> MKYNAPNTTPSSIGPQIRLDYYYKKALVDAAKEMYFGQLAEVTNMPKNMGKQIKLYHYVPLLDDRNVNDQGIDAAGATIANGNLYGSSKDIGTIPSKLPALTENGGRVNRVGFTRIQLIGSIKKFGFFYEWTQEAMDFDTDEELDSHLIQEAVKGANEITEDQLQIDLLNGAGVVRYPGAATSNADMTGEGTATVVTYEGLVKMGITLNDNLCPMQTKLIAGSLMTDTRTIQGARALYIGSELELQLRKMKDPFDNAA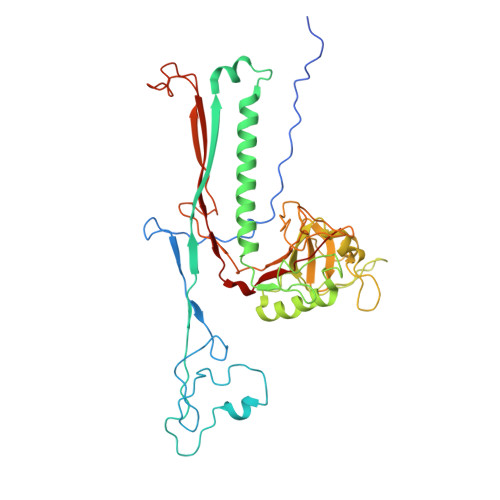FIPVQQYADAGNLLKGEIGSIASFRVIVVPKMLKWAGAGATVTTNPGYYATSGKYDVFPMLCVGSGSFTTIGFQTDGKTVKFTTYTKKPGIETVSYADPYGEMGLTSIKWYYGSLILRPEWIALFKTVAAM(9beta)-17-hydroxypregn-4-ene-3,20-dione | C21 H30 O3 | 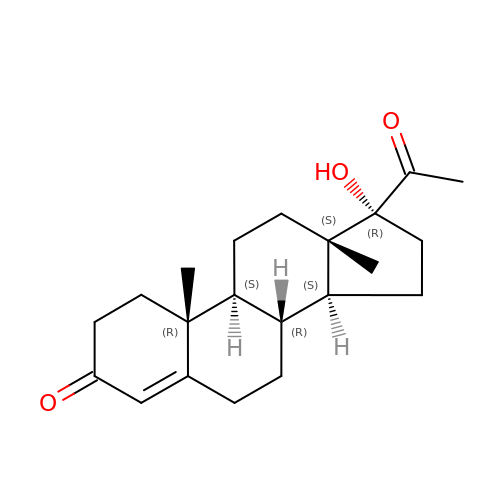DBPWSSGDRRHUNT-CEGNMAFCSA-N5-amino-1-[(3R)-1-cyanopiperidin-3-yl]-3-[4-(2,4-difluorophenoxy)phenyl]-1H-pyrazole-4-carboxamide | C22 H20 F2 N6 O2 | 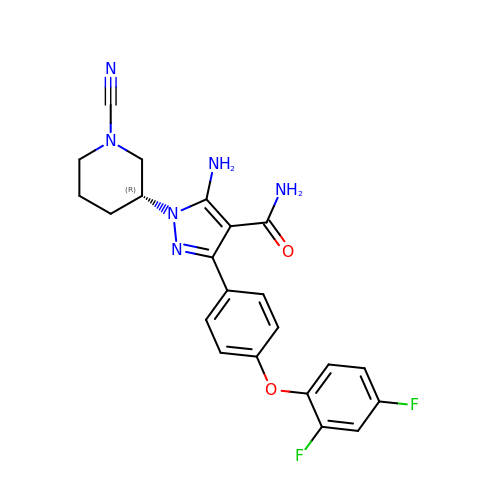SQFDBQCBXUWICP-OAHLLOKOSA-N>MDNIIMTAYISIFVQIITAIISVYGLFIPLNFKDII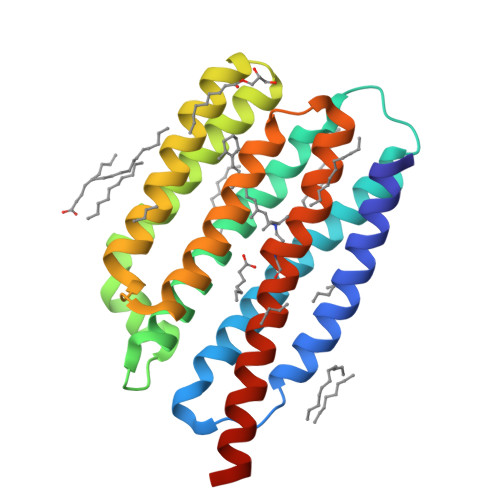LREILILELIVQIIEFIFYIWLIITLQSINEDITYVRYFDWVLTTPVMLLTTVYFFEYMNSDDGIRKKEINDRDYVYLFYICLSNFFMLLIGYLGETKQINKMLTLFGGSFFLFLTFYLLYVKYTKENWMNYIVFYFMFLVWFLYGFAFMFPFSIKNQMYNILDIVSKNIYSIFIFIVILNQSYKLLLEHHHHHH[2x]>MTYETILVERDQRVGIITLNRPQALNALNSQVMNEVTSAATELDDDPDIGAIIITGSAKAFAAGADIKEMADLTFADAFTADFFATWGKLAAVRTPTIAAVAGYALGGGCELAMMCDVLIAADTAKFGQPEIKLGVLPGMGGSQRLTRAIGKAKAMDLILTGRTMDAAEAERSGLVSRVVPADDLLTEARATATTISQMSASAARMAKEAVNRAFESSLSEGLLYERRLFHSAF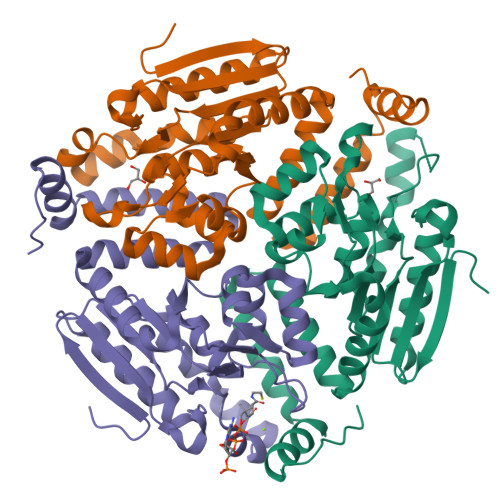ATEDQSEGMAAFIEKRAPQFTHR[6x]(3,5-di-tert-butylphenyl)boronic acid | C14 H23 B O2 | 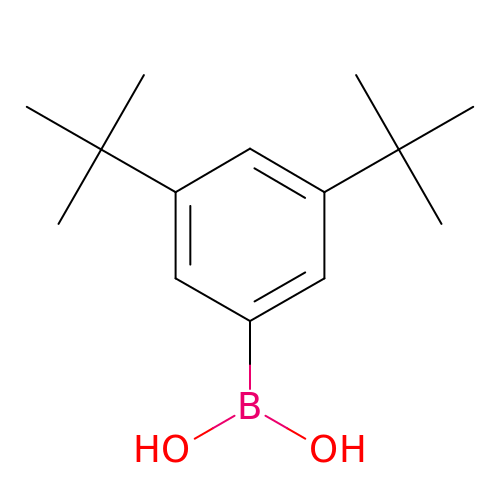RPCBIEHUQSGPNA-UHFFFAOYSA-N> MEQSVANLVDMRDVSFTRGNRCIFDNISLTVPRGKITAIMGPSGIGKTTLLRLIGGQIAPDHGEILFDGENIPAMSRSRLYTVRKRMSMLFQSGALFTDMNVFDNVAYPLREHTQLPAPLLHSTVMMKLEAVGLRGAAKLMPSELSGGMARRAALARAIALEPDLIMFDEPFVGQDPITMGVLVKLISELNSALGVTCVVVSHDVPEVLSIADHAWILADKKIVAHGSAQALQANPDPRVRQFLDGIADGPVPFRYPAGDYHADLLPGS;> MHHHHHHENLYFQSESLSWMQTGDTLALSGELDQDVLLPLWEMREEAVKGITCIDLSRVSRVDTGGLALLLHLIDLAKKQGNNVTLQGVNDKVYTLAKLYNLPADVLPR

An ABC transporter is a critical component of the Mla pathway, which is a phospholipid transport system that is important for outer membrane (OM) integrity in many Gram-negative species, and has been implicated in the Maintenance of outer membrane Lipid Asymmetry. Two copies of MlaF, an ABC ATPase, and two copies of MlaE, a multipass transmembrane protein, form an MlaF2E2 subcomplex that represents the conserved ABC transporter core. MlaB is stably associated with the cytoplasmic part of the transporter complex: one MlaB subunit binds to the side of each of the two MlaF ATPase domains. We and others have hypothesized that MlaB may regulate the MlaFEDB transporter complex, perhaps through its interaction with the MlaF ATPase. Here we report structures of the MlaFB complex, and present a model for how these two proteins may work together.

Here, we focus on the MlaF2B2 complex, which is fully assembled as expected for an ABC transporter ATPase subunit. The final model for MlaF2B2 consists of MlaF residues 5–267 (of 269 total) and MlaB residues 2–97 (of 97 total), as well as an ordered portion of the N-terminal purification tag [Prior to publication, coordinates are available for download from our website: URL]. At the core of the MlaF2B2 complex is an MlaF homodimer, assembled in a ‘head-to-tail’ arrangement similar to the NBDs of other ABC transporters in the dimeric state. Two ADP molecules are bound at the dimer interface, along with two Mg ions, representing the post-powerstroke state following ATP hydrolysis and phosphate release. Our MlaF structure adopts an open conformation capable of nucleotide exchange, with 13.9 Å separating the P-loop/Walker A motif in one subunit from the ABC signature motif in the opposing subunit (between Cα of Gly46 and Gly147). The MlaB subunits bind near the periphery of the MlaF dimer and make no direct contacts with each other. Intriguingly, each MlaF subunit possesses a unique ~25 aa C-terminal extension (CTE) that wraps around the neighboring MlaF subunit, forming a domain swapped reciprocal ‘handshake’, and interacting with the adjacent MlaB as well. Much of the C-terminal segment adopts an extended ‘random coil’ structure, before terminating in a short helix that binds to the neighboring MlaFB module, where it inserts three hydrophobic residues into a groove at the MlaF-MlaB interface (Tyr261, Leu265, Leu266). The MlaB binding site on MlaF is centered on the helical subdomain of the core NBD in MlaF, distant from the MlaF2 dimer interface and the ATP binding sites (with ~30 Å separating the nearest atoms in MlaB and the bound ADP). Binding to MlaF is mediated entirely by the helical face of MlaB, including helices α1, α2, and α3 and the C-terminal coil. α2 lies between α1 and α3, and consequently is at the center of the interface and makes the most interactions with MlaF.>GSMPPTSTTSNPIVFYDIATRPPVEKTCCSPNPW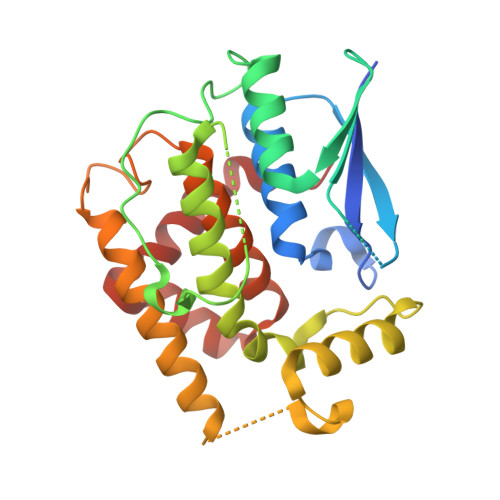KTRLALNFKDLPYSTSWVALPDISKVRGSLKVPPCRKFADGTDAFTLPIIEDPATDSLVGDSFDIAVYLQKTYPKSGAGDLFPPQSLDYVFKHNGILVPLSECRESEFPEYARFNMNIDAAFTTHTQLTVQGFPFDPATAEATKAEFVRRGGVSCWDDFALVGEQREKMMDSFQNMLGDLAKLFLKDTSGPFLLGTKASYADLMIGAWLRMMHVTLPESEWEEVRSWHEGIFGQLYDALETYAEVK[2x]> MQQLGFELSRILKQLPNLGGSDRKTRAMLLANAVALQIPFETLLDFDEQQDKAVAKFKKILSKVNENIAVDTKLAVTYFNNILRIRQSLITGITDPCLVKAVLTSDTANDY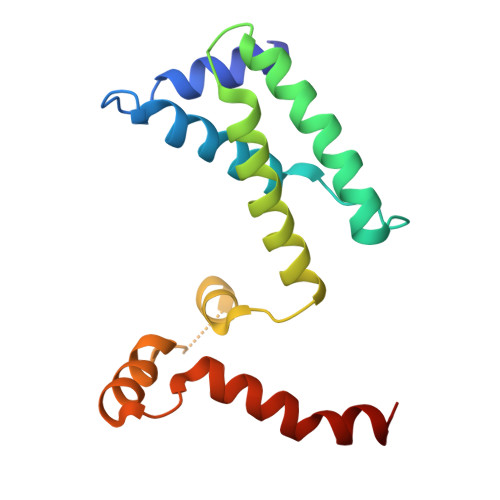LTVDDVNIVSAVVNGPDYNRIQADMGNALNQLIGSIDE>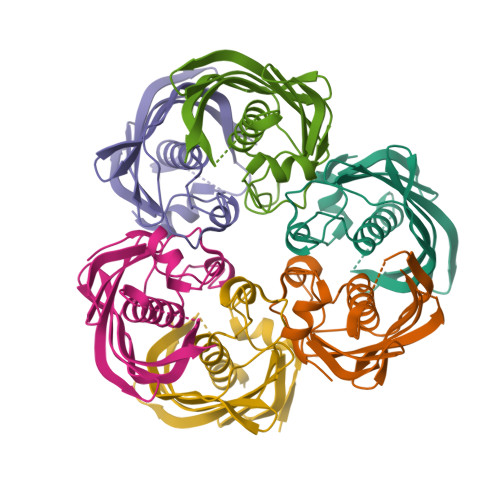[9x]MRRTIMSTEKINFDIHKILTLLPHRYPILLVDRVLELEPHKSIKALKNVTVNEPFFTGHFPKRPVMPGVLIIEALAQAAALLTFAEAEPKDPENTLYYFVGIDNARFKRVVEPGDQLILNVTFERYIRGIWKFKAVAEVDGKVAAEAELMCTVKTADAAP> GAMGSEISKTEAGQYSVSAPEHKGLVLSGGGAKGISYLGMIQALQERGKIKNLTHVSGASAGAMTASILAVGMDIKDIKKLIEGLDITKLLDNSGVGFRARGDRFRNILDVIYMMQMKKHLESVQQPIPPEQQMNYGILKQKIALYEDKLSRAGIVINNVDDIINLTKSVKDLEKLDKALNSIPTELKGAKGEQL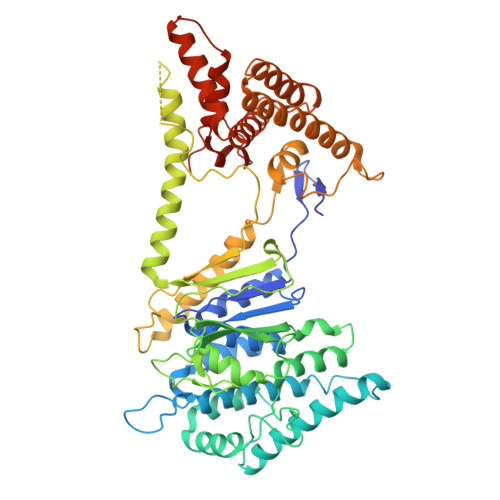ENPRLTLGDLGRLRELLPEENKHLIKNLSVVVTNQTKHELERYSEDTTPQQSIAQVVQWSGAHPVLFVPGRNAKGEYIADGGILDNMPEIEGLDREEVLCVKAEAGTAFEDRVNKAKQSAMEAISWFKARMDSLVEATIGGKWLHATSSVLNREKVYYNIDNMIYINTGEVTTTNTSPTPEQRARAVKNGYDQTMQLLDSHKQTFDHPLMAILYIGHDKLKDALIDEKSEKEIFEASAHAQAILHLQEQIVKEMNDGDYSSVQNYLDQIEDILTVDAKMDDIQKEKAFALCIKQVNFLSEGKLETYLNKVEAEAKAAAEPSWATKILNLLWAPIEWVVSLFKGPAQDFKVEVQPEP> MDDLTIEILTDDADYDLQRFDCGEEALNLFLTTHLVRQHRNKILRAYILCRNTP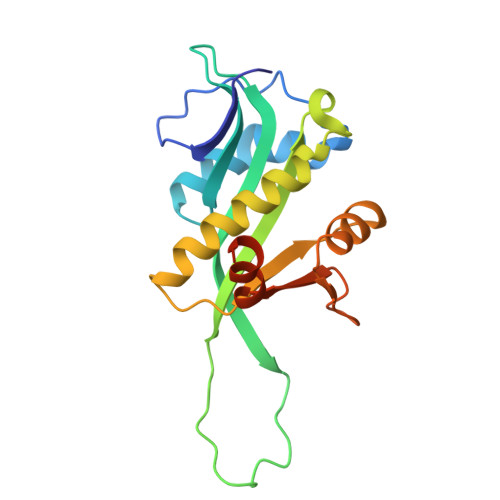ERQVLGYYTLCGSCFERAALPSKSKQKKIPYKNIPSVTLGRLAIDRSLQGQGWGATLVAHAMNVVWSASLAVGIHGLFVEALNEKAHTFYKSLGFIPLVGENENALFFPTKSIELLFTQSDLEHHHHHH2-[[(2R)-2-(3-bromanyl-5-iodanyl-phenyl)carbonyloxy-3-tetradecanoyloxy-propoxy]-oxidanyl-phosphoryl]oxyethyl-trimethyl-azanium 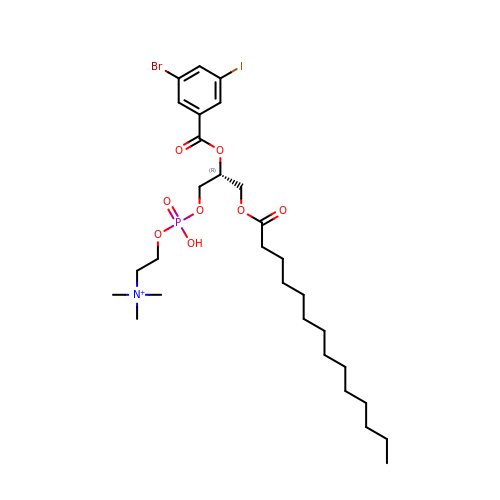| C29 H49 Br I N O8 P | RDKBFTQTYYTUKD-HHHXNRCGSA-O>[4x]MACPSQCSCSGTEVNCAGKSLASVPAGIPTTTRVLYLNSNQITKLEPGVFDRLANLRELHLWGNQLVSLPPGVFDNLANLEKLWLNSNQLTSLPAGLFDR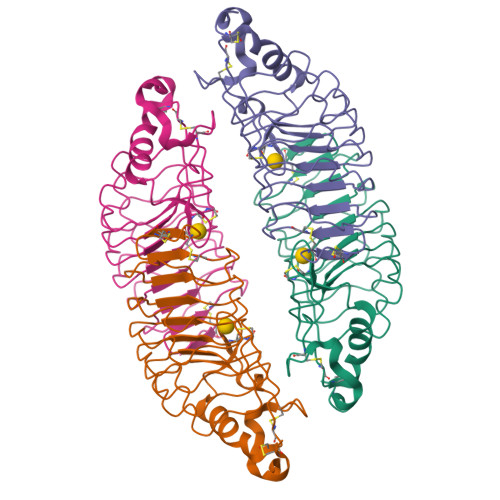LVNLEHLGLCCMKLTELPSGAFDKLTRLKQLGLDQNQLKSIPDGAFARLPSLTHVWLHTNPWDCQCTDILYLSGWVAQHSSIVGEGWPWRHSPDSAKCSGTNTPVRAVTEASTSPSKCPG>MATLAFILYKYFPFGGLQRDFMRIALECQRRGHDIRVYTLIWEGDVPDGFEVLVAPVRSIFNHRRNEKFTAWVRADLDRRPVQRVIGFNKMPGLDVYYAADACFEEKAQTLRNPLYRQWGRYRHFAGYERAVFDPASKTEILMISEVQQPLFVKHYGTQAERFHLLPPGISQDRRAPANAADVRAEFRREFGLEEDDLLLVQIGSGFKTKGLDRSLKALSALPKALRRRTRLIAIGQDDPKPFLLQIAALGLNDQVQILKGRSDIPRFLLGADLLIHPAYNENTGTVLLEALVSGLPVLVTDVCGYAHYIAEADAGRVLPSPFEQDSLNRLLAEMLEDAPARAAWSRNGLAYADHADLYSMPQRAADLILG[2x]

The glycosyltransferase WaaG in Pseudomonas aeruginosa (PaWaaG) is involved in the synthesis of the core region of lipopolysaccharides. The hexosyl sugar residue in each of the bacterial species is transferred by a glycosyltransferase (GT) referred to as WaaG to form an α-(1→3)-linkage. The PaWaaG monomer displays a typical GT-B fold, consisting of two “Rossmann-like” β/α/β domains.

In order to gain insights into substrate binding in PaWaaG we solved structures of the enzyme in complex with the nucleotide sugars UDP-glucose, UDP-galactose, and UDP-GalNAc in space group P21 to resolutions of 1.95, 2.02, and 2.20 Å, respectively. For the PaWaaG-UDP-galactose structure both monomers have unambiguous density for UDP-galactose. In PaWaaG-UDP-glucose there are three hydrogen bond interactions (Glu281, Thr283, and Asn282) which position glucose, whereas there are two additional hydrogen bond interactions (Asp19 and the backbone nitrogen of Ala99) which orient galactose and GalNAc in the PaWaaG-UDP-galactose and PaWaaG-UDP-GalNAc structures, as well as the side-chain nitrogen atom of Asn282 which is in hydrogen bonding distance (3.1 Å) to O4′ of Gal and GalNAc. Interestingly, structural comparisons show that, while the galactose portion of PaWaaG-UDP-galactose superimposes perfectly with the galactose component of GalNAc from PaWaaG-UDP-GalNAc, it occupies a quite different position to the glucose moiety of PaWaaG-UDP-glucose. In contrast to the glucose sugar comparisons, superposition of PaWaaG-UDP-galactose and PaWaaG-UDP-GalNAc with EcWaaG-UDP-2F-glucose revealed that the twisted conformation observed for glucose in PaWaaG-UDP-glucose relative to the EcWaaG structure is not present. Instead, galactose and GalNAc adopt the same overall position and orientation as 2F-glucose. The hydrogen bond networks for galactose and GalNAc are also very similar to 2F-glucose in EcWaaG. Interestingly, PaWaaG was also unable to hydrolyze UDP-galactose, despite the crystal structure showing that the sugar binds in a very similar way to GalNAc. This may be due to galactose potentially being quite mobile, as evidenced by the significant Fo-Fc peak around the anomeric carbon of the sugar, which is not observed in our PaWaaG-UDP-GalNAc structure.> SSERIRYAKWFLEHGFNIIPIDPESKKPVLKEWQKYSHEMPSDEEKQRFLKMIEEGYNYAIPGGQKGLVILDFESKEKLKAWIGESALEELCRKTLCTNTVHGGIHIYVLSNDIPPHKINPLFEENGKGIIDLQS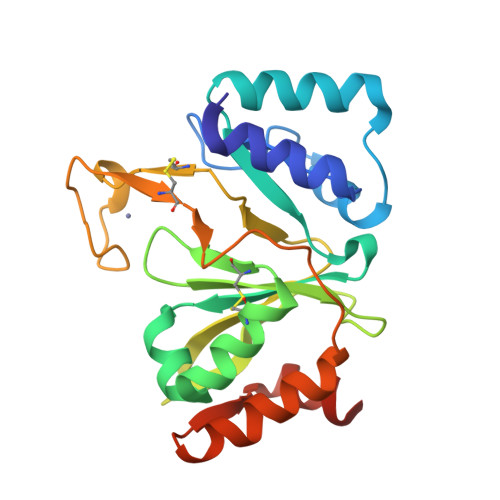YNSYVLGLGSCVNHLHCTTDKCPWKEQNYTTCYTLYNELKEISKVDLKSLLRFLAEKGKRLGITLSKTAKEWLEGHHHHHH>[3x]MVSNQQAVEQANQAKLQQQVAMGLIWTQQSGEYAALAHQAFNSAKMAFDHAKAKKGKKK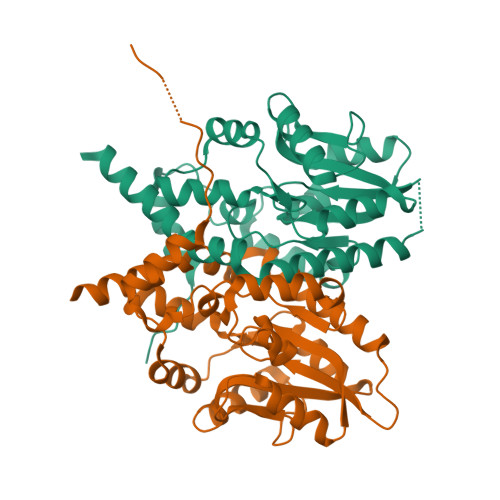AVVVDLDETMIDNSAYAGWQVQSGQGFSPKTWTKWVDARQSAAIPGAVEFSNYVNANGGTMFFVSNRRDDVEKAGTVDDMKRLGFTGVNDKTLLLKKDKSNKSVRFKQVEDMGYDIVLFVGDNLNDFGDATYKKSNAERRDFVAKNSKAFGKKFIVLPNTQYGDWEGGLDKNYFKGDSQSKLDVRAKAIHAWDGKHHHHHH>[5x]MVQTSFEHHHHHHSAGENLYFQGAQISMNIKLEIQKMAKEIGISKIGFTTADDFDYLEKSLRLGVEEGRTTGFEHKNIEERIYPKLSL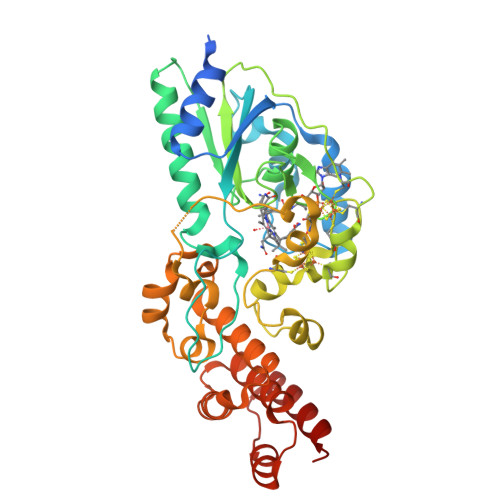ESAKTIISIAVAYPHKLPQQPQKTEFKRGKITPNSWGLDYHYVLQDKLKRLAKGIEKLTENFEYKGMVDTGALVDTAVAKRAGIGFIGKNGLVISKEYGSYMYLGELITNLEIEPDQEVDYGCGDCRRCLDACPTSCLIGDGTMNARRCLSFQTQDKGMMDMEFRKKIKTVIYGCDICQISCPYNRGIDNPLASDIDPDLAMPELLPFLELTNKSFKETFGMIAGSWRGKNILQRNAIIALANLHDRNAIVKLMEIIDKNNNPIHTATAIWALGEIVKKPDEGMLDYMRGLSPKDEHSQAEWELVCAKWQI> METYKVTKTIRFKLEAQNVPEIQKDIEGLQSEFNLANFVSDLKNYLDQVRNYLFSEGKEHVFVNNKITIKREWLQNHAKQEWVDFLEKNKRNNSLNNHTRRIQMSIGDFTGLASKIEGTFDEINSICKGLADAAGAQANKRTKRERTGLLLKRLQARKALPSLFSLIENSADKNETGNLSLQLKNKSILIEQQLAAGVQTFLPAQSGGLPVAKASFNYYTINKKPVDFGNEKSELESRLKISIDTIFKLTRENFSKKIEEAITADIQKELNNGKTLLLGDVPMLGIENYVSLRQILKNIKSNQKKAFSDLMQSGKNYNELKATNLYLLNTIEQRQFDNYKV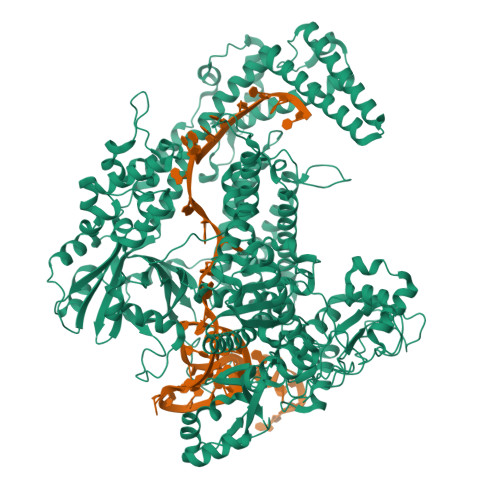KTNELEKLAVKINQATNDNQKKELISNKQRVAKQRGIIMRDNFATWKSFSNFYRTISQEHGKILALLKGIEKERTESQLLKYWALILENNGQHKLILIPREKAASCKQWIASLNPSGDKLTKLFWFESLTYRSLQKLCFGFTENGNNKFNKNIQNLLPKDNSRKIINGEFAFQGDEQKKIKFYQSVLESKYAQSVLNIPIQQVQADIINQSFASLDDFQIALEKICYRLFAVVEANIEAELLKNDKAQIFNITSSDLRKEAKDKIKSHTQIWKAFWTSENKQNNFETRLNPEITITYRQPKQSKIDKYGERSQKNNRYLHAQYTLITTISEHSNSPTKILSFMSDDEFKSSVDTFNKKFKKDEIKFAFGIDNGEVELSTLGVYFPAFDKTTYKEKVAELEKVNDYGFEVLTIRNLNYKETDYNGKERKIIQNPSYFLKKENYLRTFNKSETAYQKMFTEQFEKKKLLTLDLTTAKVICGHIVTNGDVPALFNLWLKHAQRNIFEMNDHIQKETAKKIVLKNQLDTDNEKLKFAEYISKEKEFGKLNDDEKMKYTKWIFEDRDQNNFTEVENKKFKRCQKIYGNYSTKAKAPVLFASCFIDEELQSVTDIFDVRHIFKKREDFYALKTEEEIKQLIDSYNTNRASHDISNEELDLKILNTKKALVANAVGVIDFLYKHYERRLGGEGLIIKEGFGTGKVEDGIEKFSGNIYRILERKLYQKFQNYGLVPPIKSLMAVRANGIENNKNAILQLGNVGFIDPAGTSQECPVCIEGRLEHTTTCPNKCGFNSERIMHSNDGIASFNIAKRGFNNFVKSKTDKQLEHHHHHH4-(3-methylphenyl)-6-[(1-methylpyrazol-3-yl)amino]-1~{H}-pyrrolo[2,3-b]pyridine-3-carbonitrile 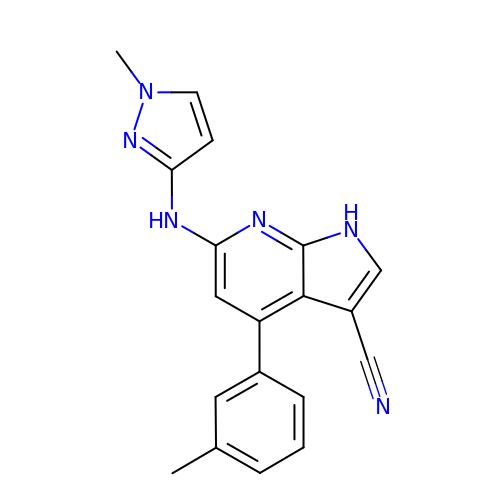| C19 H16 N6 | IQBHNQCIUDQGPV-UHFFFAOYSA-N> ANIVGGIEYSINNASLCSVGFSVTRGATKGFVTAGHCGTVNATARIGGAVVGTFAARVFPGNDRAWVSLTSAQTLLPRVANGSSFVTVRGSTEAAVGAAVCRSGRTT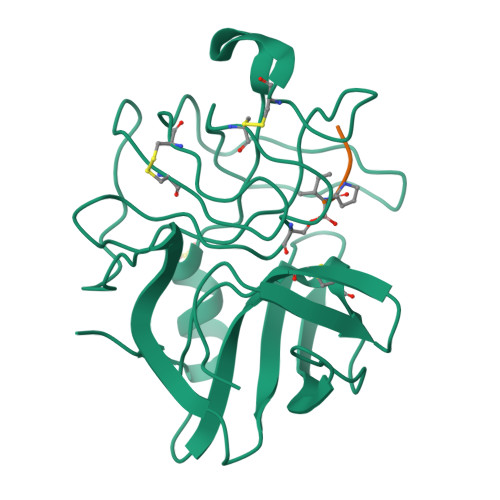GYQCGTITAKNVTANYAEGAVRGLTQGNACMGRGDSGGSWITSAGQAQGVMSGGNVQSNGNNCGIPASQRSSLFERLQPILSQYGLSLVTG;> XAAPI[METHYL(VINYL)AMINO]METHANOL | C4 H7 N O2 | 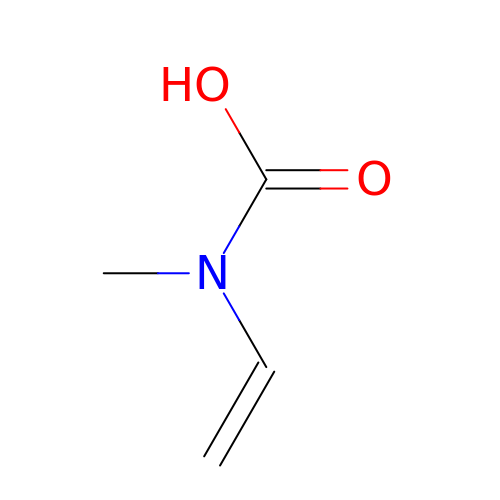RIKKDQCPYLBOND-UHFFFAOYSA-N KpsC is a dual-module glycosyltransferase (GT) essential for “group 2” capsular polysaccharide biosynthesis in Escherichia coli and other Gram-negative pathogens. Two separate GT modules in KpsC transfer 3-deoxy-β-d-manno-oct-2-ulosonic acid (β-Kdo) from cytidine-5′-monophospho-β-Kdo donor to a glycolipid acceptor. The N-terminal and C-terminal modules add alternating Kdo residues with β-(2→4) and β-(2→7) linkages, respectively, generating a conserved oligosaccharide core that is further glycosylated to produce diverse capsule structures. Based on the formation of covalent adducts with Kdo identified here by mass spectrometry and X-ray crystallography, we determined that catalytically important active site residues are conserved in WbbB and KpsC, suggesting a shared double-displacement mechanism.

To identify a more stable KpsC-NEc-Kdo adduct, an Asp160Asn variant was analyzed. However, as both a worse nucleophile and a worse leaving group, we rationalized that the resulting Kdo–Asn160 adduct would be significantly more recalcitrant to hydrolysis, allowing this intermediate species to accumulate. To determine the structure of the observed KpsC-NEc Kdo adduct, crystals of KpsC-NEc D160N were grown in the presence of 1 mM CMP before being briefly soaked in a CMP-Kdo–generating reaction mixture and then immediately frozen. In the resulting map, clear density was visible for the CMP nucleotide, which refined to an occupancy of 0.95. Additional density was associated with Asn160; this density was modeled as an α-Kdo adduct and refined to a final occupancy of 0.76, with atomic displacement parameters (B-factors) similar to surrounding residues. This adduct was modeled as being linked to the Oγ of Asn160. Finally, a less defined density peak stacked on Trp42 was modeled as a Kdo residue with partial occupancy (0.78). The α-Kdo adduct is stabilized in the active site by an extensive network of hydrogen bond interactions, mediated by a series of highly conserved residues. The observed binding mode places the exocyclic O7 and O8 nearest the CMP phosphate group, while the anomeric carbon is positioned 5.4 Å away. Nevertheless, the distance between the anomeric carbon and the CMP phosphate suggests that the adduct undergoes significant structural rearrangement after transfer of Kdo from CMP.

> MGIGIYSPGIWRIPHLEKFLAQPCQKLSLLRPVPQEVNAIAVWGHRPSAAKPVAIAKAAGKPVIRLEDGFVRSLDLGVNGEPPLSLVVDDCGIYYDASKPSALEKLVQDKAGNTALISQAREAMHTIVTGDMSKYNLAPAFVADESERTNIVLVVDQTFNNMSVTYGNAGPHEFAAMLEAAMAENPQAEIWVKVHPDVLEGKKTGYFADLRATQRVRLIAENVSPQSLLRHVSRVYVVTSQYGFEALLAGKPVTCFGQPWYASWGLTDDRHPQSALLSARRGSATLEELFAAAYLRYCRYIDPQTGEVSDLFTVLQWLQLQRRHHHHHH>[2x]MSENKATLMEGMTEKTLHSPNTMAEVASLHVAN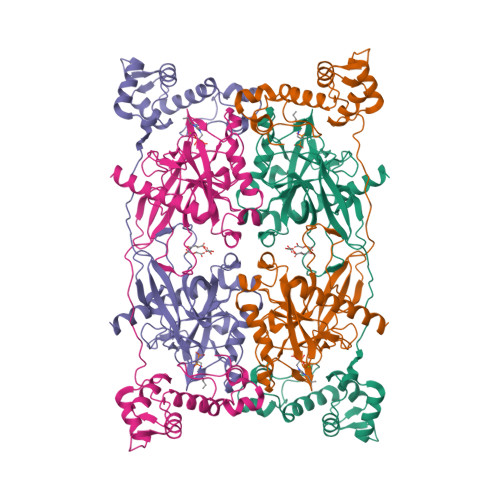SYIGTGLDTSLENVKPLPEACKRNVTEFDLVAYGKDEFTLSMEKRVMARMFSAFDVTQLGYLEERKIEHMCKYLGRVMNEDDVKQMKSEINAIDGHITFEKFWAWWCSHPEVPAKKDFFSMVSVDFAVPYHQQQLLTRETGELYTPSYRVLYYFRDMETGKELQVSPWHDIPLYVRDLVRTKPASLPMNRYNFICEIPKWTRAKFEIATGEPFNPIKQDIKNGVPRFYKHGDMMWNYGALPQTWESTDVVFEGGYVGDNDPIDAIEIGMTQFKVGQVGAVKVLGILGMIDDGQMDWKVICISHNDPICRFLKDIHDVPKFLPGCLDAIHEWFRVYKICQGGVENKFVFNGEFKDKSFAMKVIDESHYMWGNLRKINKKEEV The bacterial Rho factor is a ring-shaped motor triggering genome-wide transcription termination and R-loop dissociation. Rho is essential in many species, including in Mycobacterium tuberculosis where rho gene inactivation leads to rapid death. Yet, the M. tuberculosis Rho [MtbRho] factor displays poor NTPase and helicase activities, and resistance to the natural Rho inhibitor bicyclomycin [BCM] that remain unexplained. Since Rho has no structural homologs in eukaryotes, it is an attractive target candidate for the development of new antibiotics.

Moreover, the analysis of the closed ring dataset did not permit to compute a reliable and interpretable map, while particles corresponding to the open conformation allowed us to compute a cryo-EM map at 3.3 Å resolution (which led to the structure of the hexamer in the open ring conformation), showing an open-ring organization of the complex resulting from the assembly of six MtbRho subunits. The MtbRho is composed of six subunits adopting an open corkscrew conformation. The N-termini, including NIDs, are not resolved in the structure of the MtbRho hexamer. The presence of a clear electron density in all the ATPase pockets of MtbRho reveals that ATP ligands are held by a network of interactions involving the phosphate, sugar, and adenine base moieties. The adenine base is stacked on Phe530 while Thr333 and Thr361 form hydrogen bonds with the NH2 and N7 groups of adenine, respectively. These H-bonds explain the marked preference of MtbRho for purine versus pyrimidine triphosphates. Consistent with the open configuration of the MtbRho ring and the absence of activating RNA ligand, the ATPase pockets are in an unproductive state. Furthermore, the arginine valve (R387) and catalytic glutamate (E386) residues are too distant from, respectively, the γ-phosphate and catalytic Mg2+ ion to catalyze ATP hydrolysis. However, close inspection of the BCM-binding cavity in our MtbRho structure revealed that it contains a methionine (Met495) instead of a leucine (Leu320) in EcRho. This Leu→Met substitution creates a bulk in an otherwise structurally comparable cavity, which could penalize BCM binding by steric clash.

>[6x]MGSSHHHHHHSSGLVPRGSHVTDTDLITAGESTDGKPSDAAATDPPDLNADEPAGSLATMVLPELRALANRAGVKGTSGMRKNELIAAIEEIRRQANGAPAVDRSAQEHDKGDRPPSSEAPATQGEQTPTEQIDSQSQQVRPERRSATREAGPSGSGERAGTAADDTDNRQGGQQDAKTEERGTDAGGDQGGDQQASGGQQARGDEDGEARQGRRGRRFRDRRRRGERSGDGAEAELREDDVVQPVAGILDVLDNYAFVRTSGYLPGPHDVYVSMNMVRKNGMRRGDAVTGAVRVPKEGEQPNQRQKFNPLVRLDSINGGSVEDAKKRPEFGKLTPLYPNQRLRLETSTERLTTRVIDLIMPIGKGQRALIVSPPKAGKTTILQDIANAITRNNPECHLMVVLVDERPEEVTDMQRSVKGEVIASTFDRPPSDHTSVAELAIERAKRLVEQGKDVVVLLDSITRLGRAYNNASPASGRILSGGVDSTALYPPKRFLGAARNIEEGGSLTIIATAMVETGSTGDTVIFEEFKGTGNAELKLDRKIAERRVFPAVDVNPSGTRKDELLLSPDEFAIVHKLRRVLSGLDSHQAIDLLMSQLRKTKNNYEFLVQVSKTTPGSMDSD>[4x]RLFGTAGIRGTLWEKVTPELAMKVGMAVGTYKSGKALVGRDGRTSSVMLKNAMISGLLSTGMEVLDADLIPTPALAWGTRKLADAGVMITASHNPPTDNGVKVFNGDGTEFYVEQERGLEEIIFSGNFRKARWDEIKPVRNVEVIPDYINAVLDFVGHETNLKVLYDGANGAGSLVAPYLLREMGAKVLSVNAHVDGHFPGRKPEPRYENIAYLGKLVRELGVDLAIAQDGDADRIAVFDEKGNYVDEDTVIALFAKLYVEEHGGGTVVVSIDTGSRIDAVVERAGGRVVRIPLGQPHDGIKRYKAIFAAEPWKLVHPKFGPWIDPFVTMGLLIKLIDENGPLSELVKEIPTYYLKKANVLCPDEYKAEVVRRAAEEVERKLSSEIKEVLTISGFRIALNDGSWILIRPSGTEPKIRVVAEAPTEKRRDELFEMAYSTVSRIVKEAEKK

Thermococcus kodakarensis, a hyperthermophilic archaeon, harbors a novel enzyme (PPMTk) that exhibits high homology with phosphohexomutases but has no significant phosphohexomutase activity. Instead, PPMTk catalyzes the interconversion of ribose 1-phosphate and ribose 5-phosphate. It contains the active site motif, “TXSHNP” (serine as the active site residue), and “DXDXDR” (the metal-binding site) conserved in various phosphohexomutases. Thermostability analysis has revealed that PPMTk is highly stable at higher temperatures with a half-life of 90 min at 100 °C.

To understand this unique property, we crystallized PPMTk and determined the three-dimensional structure by X-ray diffraction at a resolution of 2.39 Å. Crystals of PPMTk were grown in 7 days as needles (0.1 mm long) in a monoclinic space group P21 with four protomers in the asymmetric unit. The structure was found to be a homotetramer. The crystal structure of PPMTk contains two monomer–monomer, and one dimer–dimer interfaces stabilized by H-bonds and salt bridges. The protomer was composed of two main domains, the N-terminal domain consisting of residues 1-350 and the C-terminal domain formed by residues 355-450. The two domains were linked via a short linker (loop 26) forming a deep cleft. Domains I, II, and III consist of a three-layer α/β/α sandwich each, while domain IV has a two-layer α/β sandwich topology. The N-terminal domain of PPMTk was characterized by low-to-moderate B-factors resulting from stabilizing interactions between domains from different protomers within the tetramer. C-terminal domains, however, were not significantly stabilized by interactions with other domains. As a consequence, their B-factors were high and their coordinates were less well-defined.> SPPKRLTREAMRNYLKERGDQTVLILHAKVAQKSYGNEKRFFCPPPCVYLMGSGWKKKKEQMERDGCSEQESQPCAFIGIGNSDQEMQQLNLEGKNYCTAKTLYISDSDKRKHFMLSVKMFYGNSDDIGVFLSKRIKVISKPSKKKQSLKNADLCIASGTKVALFNRLRSQTVSTRYLHVEGGNFHASSQQWGAFYIHLLDDDESEGEEFTVRDGYIHYGQTVKLVCSVTGMALPRLIIRKVDKQTALLDADDPVSQLHKCAFYLKDTERMYLCLSQERIIQFQATPCPKEQNKEMINDGASWTIISTDKAEYTFYEGMGPVLAPVTPVPVVESLQLN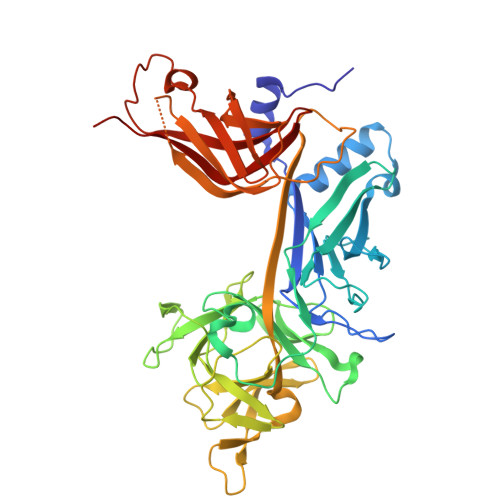GGGDVAMLELTGQNFTPNLRVWFGDVEAETMYRCGESMLCVVPDISAFREGWRWVRQPVQVPVTLVRNDGVIYSTSLTFTYTPEP> SVA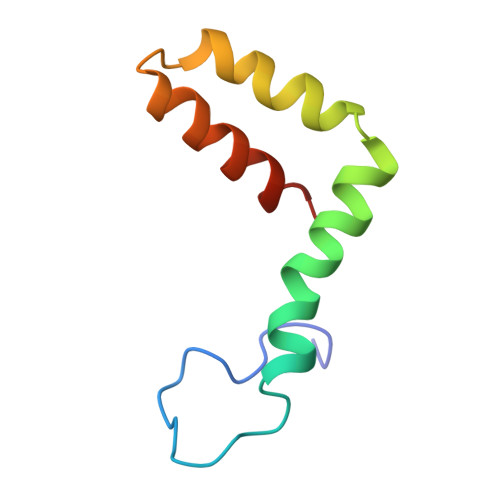LVPHVGMGLETATETWMSSEGAWKHAQRIETWILRHPGFTIMAAILAYTIGTTHFQRALIFILLTAVAPSMT> GAMAPVTEKDLAEDAPWKKIQQNTFTRWCNEHLKCVNKRIGNLQTDLSDGLRLIALLEVLSQKRMYRKYHQRPTFRQMQLENVSVALEFLDRESIKLVSIDSKAIVDGNLKLILGLVWTLILHYSISMPVWEDEGDDDAKKQTPKQRLLGWIQNKIPY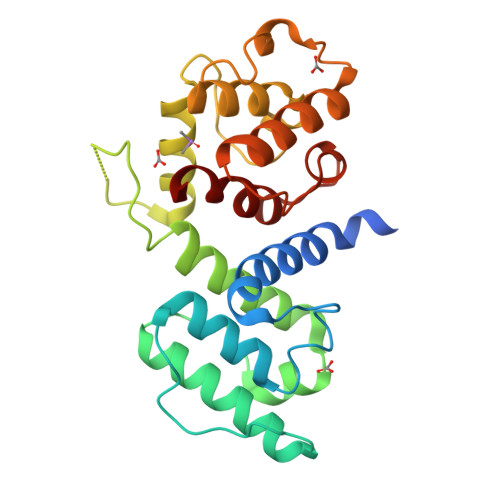LPITNFNQNWQDGKALGALVDSCAPGLCPDWESWDPQKPVDNAREAVQQADDWLGVPQVITPEEIIHPDVDEHSVMTYLSQFPKAKL>MAIETNAVVITDLNPLYPRDRDYIYEGAAQIRLIKQTLQNTFPNVTEPVDIDSDTFKIMSEKLKFTGDAMDVGGLMIKNVTPGTGDKDVVTKGQMEAFMKNWMENKLYRIGSYYITEEDINPGDSISLGFGSWAKVTGVIMGTGVVNPDGSVPNAQRVEFQAGGTGGRVFNTIRTENVPLMTVNGSSFSLSSNTHSHNMVFGRGDASGHNSSPNWYSPGGGYSQRTDNDTHTHTISGSVSLGRDDISRQPINTLPPFRAAHIWRRIS[3x];>MIVYNNQAPDAVNNVGQFGATEGSIGAYKQAAEYAADSKYWALLAESKFGTIDDLIAEVERLYQQGVLMKQDIEDLKQDFKDQDARLMSLIAQTNAAVSDANNAVALINQKLIEVQNQLDVLLGMSVDVTTLPPGTPATGSFNPNTGVISLGIPEGEPGKDGSVKDLDTAPTGVPELGDLGFYVDKDDNTVHKTTLENIANLTPSVRSVSVNGGPALDGEVALTINKETVGLGNVLNVAQYSRQEINDKFDKTTKTYQSKAEAYADAQYRQVGEKVLVWEATKYEFYTVAANKTLTPVKTEGRILTVNSRSPDSSGNIDITIPTGNPSLYLGEMVMFPYDPSKNISYPGVLPADGRLVSKESASDLGPSLVSGQLPVVSETEWQSGAKQYFSWGKLADGITDADSTNFINIRLPDWTGGEAIRAPDSDKDSQYNGSVQAQKPYVVTVNNQAPDEITGNVNISRSILGAASSGANSDITSLSGLTTPLSISQGGTGAKDAASARSNLGLGSVSTLDNVPIASGGTGAGDAAGARFNLGLGNSATMNTGTNSDNVLKVGDFGIGRPDGALVFDTTSQDQLLAGLDTYGLCVFRNNQQIAAPWDIWNYSSNLFFRAGDTYSMISIPFESAGKIKVFGGASGSGWKTSRTVYDTVNTTVDVNGFIKAASPIVKVFHDGSFETNEQSDGVSVKKISTGVYLISGCLGLNSDAGWGGVDGGFEIPIDRNKQPRVWLDYEVKEDGSLLIKTYHRTHSTSPAFARNELEGFSDGDPVDIPKDAFISVRVEMPSK[3x];> MALYPIKSLGAVGVIADQAPTDLAPNAFTNAINARFVEQRVFKTGGNAPLSYVDEDKDLTPLSFVSMPFDYYSAGNSFLVVGTNKKLYKLTDESLTDISRKVATVTKKASASIKIYPVVSQIVPKESTISMNFNQTKNLEVSLLPADANNTNLIWEVSNSSYGSITVDPSDSKLATLTSFEKEGNLVVTISTANESVVAQIAVNIIDGDSGIFLSQDTVTIRKGGTTTLTAVTGKTPVTWSSNNASIVSVTPNANSLTAVITANGEGNVTITADNGTKTASCEIVSIPQIDSISLSQSDVTVSRGSQYILTATLSPANAPNQNITWTSSNPNIATVSGTSTQGTINALLAGFTEITATTEEGNRVAVCTVRVDLAGRTMRTSAMAFAAPVSESVETQEEEVVTPPESEETVYFAEPTSGIDTSGMYEGNNFYDYSNVNDIEGFARASLLATPLSSVTLDIVSASLDVGEEIVITATASPEGEYSYQWSVDKTGYVSTTSVTGKSIKLVALRKGEINVTCTVSQMTQKDYDAFDDYPWYHAVISNCAVATTHYETPQVKEFESEYFVDLPGWGEQTVVDNDGNPSVKKFNWKCERVRSFNNRLFALNMREANASGVTTNYPLRLRWSNFANENKAPTLWDDFAYDRVVSSDLASNIVGQTQALENGYAGYIDLADSNGSLIDILPLKDYLFVYTEFETYIGSPTNNTYQPLMFKKLFNDSGILAPECVVEVEGSHFVVTQNDVILHNGATKKSIASNRVKNMLINEVCLVNPLATRVHLHQDKKEVWVLYVGPGEPKESFACTKAAVWNYEFDTWSFRTIPYAQCIGLVDPPVLERGPIWSDFQEITWDDPSIKELVWRKDATNFRQRVTIVGSFLKGFYQVDVGALDYFYDRLNDVVIEKPLEMRLERTGIDFDNVTNEWNQKHINRFRPQTTGSGTYIFEAGGSQFSNEYGHPHTSKTYTIGVD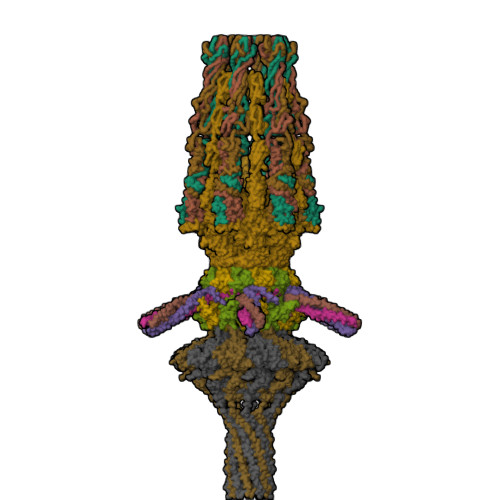RHVSVRLNHPYLFYNVIDNDVNSNAAINGLTIEFAVGGRR;>MAMPDVQYPINTYGWLKKAVALWADRDDDEFVNQIPNFINFAEKEIYRNLRIPPLEKEVYLDIKDGVAYIPPDYLEAQWMMRAKDGTIFQVTSPEEISYRRQHGTINPSHWNNQPVNFARFGSRFIFYPSIEADTPYYPDDGSPLIPAENSVILSYYADPPEFHEDTDTSTILTIAPELLLYFTLRHACLFVQDDNGVQKWSALGKAILDEMVEQNKKQEYSGSPIAIPNNMTRLQSSLPDIYGIRTSRV[2x];>[2x]MAKQKYSEEVLDELRVDLQRRFNYAQGYVDMAVKGYAREAWEYFYGNLPAPVTAGSSSWVDRTVWESVNGTLQDIINVFCSGDEAVTFVADNQQDSDAADVATKLVNQILLRDNPGYNIISSAAQECLVTRNSFIKYYWDEQTSTQTEEAEGVPPEALAAYVQGLEAGGLKNLEVFTEENEDGTVDVKVTYEQTVKRVKVEYVPSEQIFVDEHATSFADAQYFCHRVRRSKEDLVAMGFPKDEIEAFNDWTDTMDTTQSTVAWSRTDWRQDIDADIGTDTEDIASMVWVYEHYIRTGVLDKNKESKLYQVIQAGEHILHTEEVTHIPFVTFCPYPIPGSFYGQSVYDITKDIQDLRTALVRGYIDNVNNANYGRYKALVGAYDRRSLLDNRPGGVVEMERQDAIDLFPYHNLPQGIDGLLGMSEELKETRTGVTKLGMGINPDVFKNDNAYATVGLMMNAAQNRLRMVCRNIAHNGMVELMRGIYNLIRENGEVPIEVQTPRGMIQVNPKQLPARHNLQVVVAISPNEKAERAQKLISLKQLIAADAQLAPLFGLEQDRYMTAQIFELMGIKDTHKYLLPLEQYQPPEPSPMEILQLEMTKAQVENVQASSQKMIADAFDQRERTTFEQQKAADELSLRQEELQFKQENAADAMTLENRKEDNNATLEQAKHKLALMQQQVRQYESVLKELQMVMSHQVDQEKIVQQARVQDKTLELQKKEANVTKKEQQASLKDSRIPGKRLGSKK> GPGRPQESLSLVDASWELVDPTPDLQALFVQFNDQFFWGQLEAVEVKWSVRMTLCAGICSYEGKGGMCSIRLSEPLLKLRPRKDLVETLLHEMIHAYLFVTNNDKDREGHGPEFCKHMHRINSLTGANITVYHTFHDEVDEYRRHWWRCNGPCQHRPPYYGYVKRATNREPSA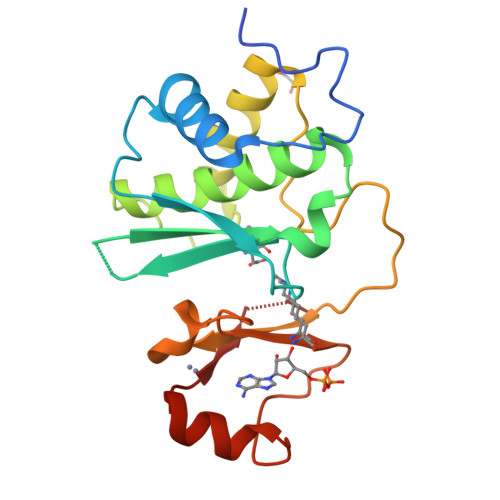HDYWWAEHQKTCGGTYIKIKE>GAMGSMEGSPSLRRMTVMREKGRRQAVRGPAFMFNDRGTSLTAEEERFLDAAEYGNIPVVRKMLEESKTLNVNCVDYMGQNALQLAVGNEHLEVTELLLKKENLARIGDALLLAISKGYVRIVEAILNHPGFAASKRLTLSPCEQELQDDDFYAYDEDGTRFSPDITPIILAAHCQKYEVVHMLLMKGARIERPHDYFCKCGDCMEKQRHDSFSHSRSRINAYKGLASPAYLSLSSEDPVLTALELSNELAKLANIEKEFKNDYRKLSMQCKDFVVGVLDLCRDSEEVEAILNGDLESAEPLEVHRHKASLSRVKLAIKYEVKKFVAHPNCQQQLLTIWYENLSGLREQTIAIKCLVVLVVALGLPFLAIGYWIAPCSRLGKILRSPFMKFVAHAASFIIFLGLLVFNASDRFEGITTLPNITVTDYPKQIFRVKTTQFTWTEMLIMVWVLGMMWSECKELWLEGPREYILQLWNVLDFGMLSIFIAAFTARFLAFLQATKAQQYVDSYVQESDLSEVTLPPEIQYFTYARDKWLPSDPQIISEGLYAIAVVLSFSRIAYILPANESFGPLQISLGRTVKDIFKFMVLFIMVFFAFMIGMFILYSYYLGAKVNAAFTTVEESFKTLFWSIFGLSEVTSVVLKYDHKFIENIGYVLYGIYNVTMVVVLLNMLIAMINSSYQEIEDDSDVEWKFARSKLWLSYFDDGKTLPPPFSLVPSPKSFVYFIMRIVNFPKCRRRRLQKDIEMGMGNSKSRLNLFTQSNSRVFESHSFNSILNQPTRYQQIMKRLIKRYVLKAQVDKENDEVNEGELKEIKQDISSLR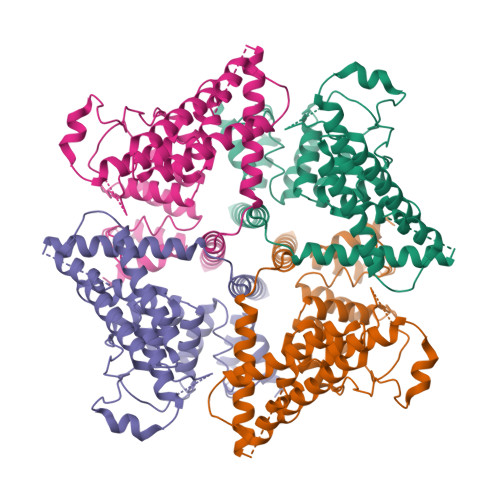YELLEDKSQATEELAILIHKLSEKLNPSMLRCE[4x]>[3x]MITAQAVLYTQHGEPKDVLFTQSFEIDDDNLAPNEVIVKTLGSPVNPSDINQIQGVNPSKPAKTTGFGTTEPAAPCGNEGLFEVIKVGSNVSSLEAGDWVIPSHVNFGTWRTHALGNDDDFIKLPNPAQSKANGKPNGLTINQGATISVNPLTAYLMLTHYVKLTPGKDWFIQNGGTSAVGKYASQIGKLLNFNSISVIRDRPNLDEVVASLKELGATQVITEDQNNSREFGPTIKEWIKQSGGEAKLA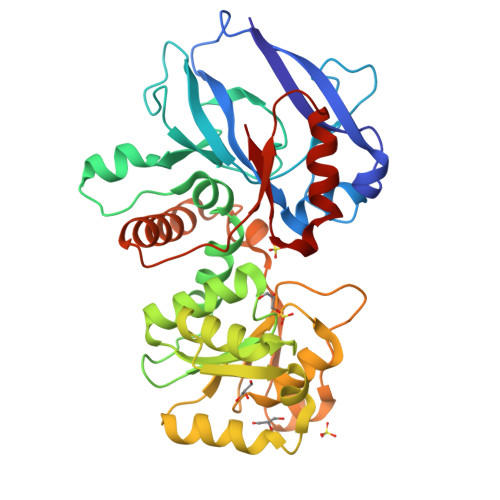LNCVGGKSSTGIARKLNNNGLMLTYGGMSFQPVTIPTSLYIFKNFTSAGFWVTELLKNNKELKTSTLNQIIAWYEEGKLTDAKSIETLYDGTKPLHELYQDGVANSKDGKQLITY>[8x]SHAGANDLCQECEDIVHLLTKMTKEDAFQEAIRKFLEQECDILPLKLLVPRCRQVLDV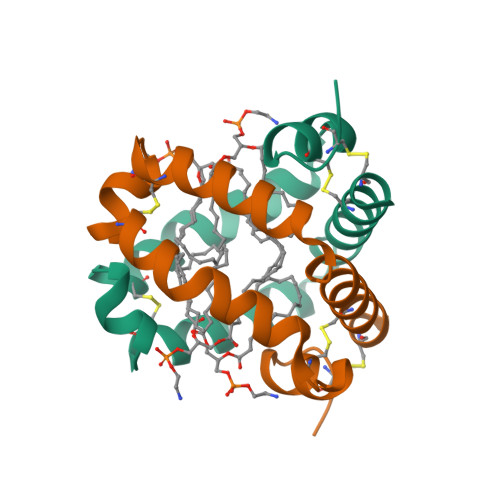YLPLVIDYFQSQINPKAICNHVGLCPRGQ>MTHPSGEPVYADAVLNGWLTSMGLGVEYVRAEGNTVYYLDDEGREVPVLDHACGFGSLIFGHNHPEIIAHAKAALDAGTVVHAQLSRQPRANQISRILNDIMRRETGRDDRYNAIFANSGAEANEICMKHAELERQERITALFAEIDAELDTAREALTTGTATLDTASLPLVGGGAGDVDGVIADIHRHNDERRAERPLFLTLDGSFHGKLVGSIQLTQNEPWRTPFTALSSPARFLPADEPELIGKIVEDERRSVLTLSLDKDTVRVVERDFPVVAAIFVEPVRGGSGMKTVTPELAEELHRLRDTLGCPLVVDEVQTGIGRTGAFFGSALLGIRGDYYTLAKAIGGGIVKNSVALIRQDRFLPAMEVIHSSTFAKDGLSASIALKVLEMVEADGGRVYQRVRERGQRLEAMLESVRADHSDVVSAVWGTGLMLALELRDQSNATSQAIREKAAHGFLGYVLAGFLLREHHIRVLPAGPRSGFLRFSPSLYITDEEIDRTETALRSLFTALRDQDGDRLVLS[4x]

Previously, the biosynthetic pathway of the immunosuppressive agent caerulomycin A (CRM A) from the marine actinomycete Actinoalloteichus cyanogriseus WH1-2216-6 has been identified, and the critical role of the (S)-selective ω-transaminase CrmG in the biosynthesis of CRM A has been reported. CrmG catalyzes amino acceptor caerulomycin M (CRM M) transformation to caerulomycin N (CRM N). Moreover, the activity of CrmG is insensitive to inhibition from ketone α-ketoglutarate or pyruvate.

The crystal structures of CrmG in complex with amino donor l-Gln, l-Glu, or l-Ala in P1 space group were determined to resolution 2.35, 2.25, and 2.20 Å, respectively. For these three crystal structures, each asymmetric unit contains two dimers. In the structures of CrmG with l-Glu or l-Ala, clear electron density was observed between the N atoms of those amino donors and the C4′ atom of PLP, indicating that we have captured the external aldimine for these amino acids. In the structure of CrmG with PLP-Ala, due to the shorter side chain and lack of γ-carboxylate or γ-carboxamide group, the l-Ala portion only forms contact with residues of R486 and Q318 from one monomer via salt bridge and hydrogen bond interaction, respectively, without interacting with the second monomer of CrmG dimer. Similarly, in the structure of CrmG in complex with l-Ala (corresponding amino donor for by-product pyruvate), the carboxyl group of l-Ala forms a hydrogen bond with Q318 and a salt bridge with R486. However, CrmG is insensitive to pyruvate inhibition with Ki of 225.9 mM. Based on these three crystal structures, amino donors l-Glu, l-Gln, and l-Ala exhibit strong, moderate, and weak binding to CrmG, respectively, due to side chain differences. These corroborate well with our kinetic data that, Km value for l-Glu, l-Gln, and l-Ala toward CrmG is 80.02, 182.70, and 405.10 μM, respectively. With amino donor l-Ala, 50% conversion of CRM M to CRM N was achieved in 48 h.> GSHMLSDEQMQIINSLVEA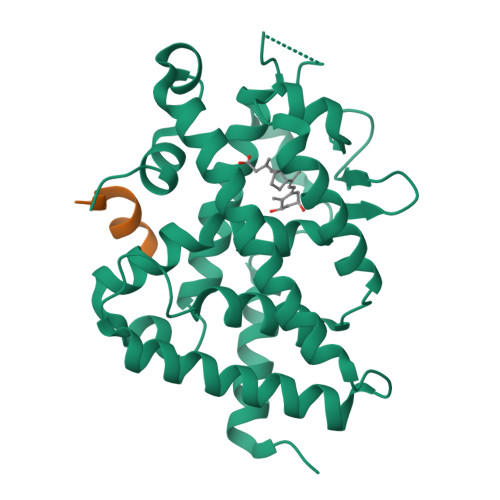HHKTYDDSYSDFVRFRPPVRVGPVTRSASRAASLHSLSDASSDSFNHSPESVDTKLNFSNLLMMYQDSGSPDSSEEDQQSRLSMLPHLADLVSYSIQKVIGFAKMIPGFRDLTAEDQIALLKSSAIEIIMLRSNQSFSLEDMSWSCGGPDFKYCINDVTKAGHTLELLEPLVKFQVGLKKLKLHEEEHVLLMAICLLSPDRPGVQDHVRIEALQDRLCDVLQAYIRIQHPGGRLLYAKMIQKLADLRSLNEEHSKQYRSLSFQPEHSMQLTPLVLEVFGSEVS;> NHPMLMNLLK Mirolysin is a secretory protease of Tannerella forsythia, a member of the dysbiotic oral microbiota responsible for periodontitis. T. forsythia secretes a family of six multidomain proteases: three serine proteases (mirolase, miropsin-1, and miropsin-2) and three metalloproteases (karilysin, mirolysin, and forsilysin), referred to as KLIKK proteases. Mirolysin, together with other M43B proteases, archetypal ulilysin and human pappalysins (pregnancy-associated plasma proteases) that hydrolyse growth hormone-binding proteins, shares unique specificity for Xaa–Arg and Xaa–Lys (P1–P1′) peptide bonds, and thus is dubbed LysargiNase17. In this study, we show that mirolysin latency is achieved by a “cysteine-switch” mechanism exerted by Cys23 in the N-terminal profragment.

To determine the molecular mechanism of the interaction of cpd 9 with mirolysin, the crystal structure of the inhibitory complex was solved. The obtained data allowed us to solve the structure in the P1 space group, representing six protein molecules in the asymmetric unit. All molecules show evidence of bound cpd 9, represented by electron density in the difference electron-density map (Fo – Fc) close to the active site of the enzyme. Although the coverage of the fragments by electron density differs for the different protein molecules in the presented structure, unambiguous placement of cpd 9 was achieved for each protein molecule in the unit cell. Cpd 9 is inserted deep in the S1′ subsite of the substrate-binding pocket formed by Asp94, Leu181, Tyr216, Arg220, Thr221, His224, Tyr286, Thr287, and Met292. The main binding contributions come from a hydrogen bond between the backbone carbonyl of Thr287 and the primary amine of cpd 9, water-mediated interaction of the cpd 9 primary amine and the Asp289 side chain, and π–π stacking interactions of the Tyr286 side chain and the ring system of the fragment, as well as π–alkyl interaction of Leu181 with the same moiety of cpd 9. As in the case of the product complex of mature mirolysin, Lys at P1′20, the amino group of cpd 9 interacts with Thr287 and Asp289 at the bottom of the S1′ pocket, but additionally, the aromatic ring of cpd 9 interacts with Leu181 and Tyr286 in the walls forming the S1′ subsite. However, in stark contrast to Arg and Lys side chains, cpd 9 does not contain an aliphatic straight-chain, aside from the amine group, but instead contains an aromatic ring, which fits well into the deep and spacious S1′ subsite in the mirolysin substrate-binding pocket. Cpd 9 and cpd 10 inhibited mirolysin with a Ki of 3.2 and 22 µM, respectively.

>RSVPSSTILIPVVVHVVYNNSAQNISDAQIISQIQVLNEDFRRMNADQANTPSAFANLAGNANIEFKLARRDPNGNTTNGITRTSTSTETFSMEMDNVKFSNLGGNNAWNTRRYLNIWVCNLGDDLLGYAQFPFEFQTKPNTDGVVIHYKHFGRDGSAESPYDKGRTATHEVGHWLDLRHIWGDDGGSCSGTDNIADTPNQGGYNEGCPSFPKTDHCTNTSPGVMFMNYMDYTYDACMNLFTKGQVERMRSLFDTQTGIRREMQIYANELTNPLSFS[6x]(E)-4-(1-(4-(1-cyclopropylpiperidin-4-yl)phenyl)-5-hydroxy-2-phenylpent-1-en-1-yl)phenol | C31 H35 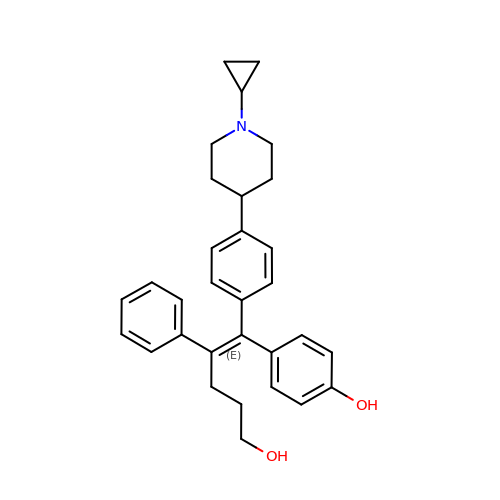N O2 | QLPDYHPRQYYVTE-NVQSTNCTSA-N>[2x]GAMQGEVSKAASADSTTEGTPADGFTVLSTKSLFLGQK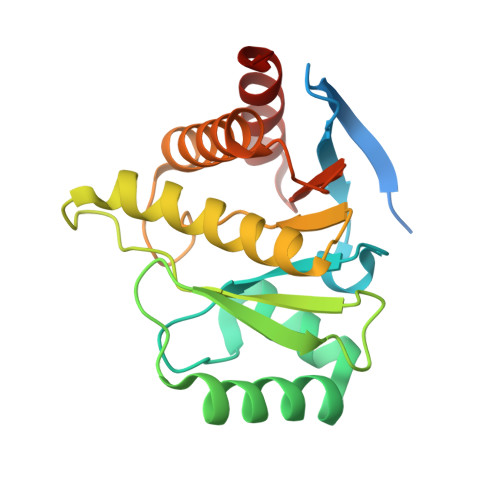LQVVQADIASIDSDAVVHPTNTDFYIGGEVGNTLEKKGGKEFVEAVLELRKKNGPLEVAGAAVSAGHGLPAKFVIHCNSPVWGADKCEELLEKTVKNCLALADDKKLKSIAFPSIGSGRNGFPKQTAAQLILKAISSYFVSTMSSSIKTVYFVLFDSESIGIYVQEMAKLDAN>MSQSNRELVVDFLSYKLSQKGYSWSQFSDVEENRTEAPEGTESEAVKQALREAGDEFELRYRRAFSDLTSQLHITPGTAYQSFEQVVNELFRDGVNWGRIVAFFSFGGALCVESVDKEMQVLVSRIAAWMATYLNDHLEPWIQENGGWDTFVELYGNNAAAESRKGQERLEGGMA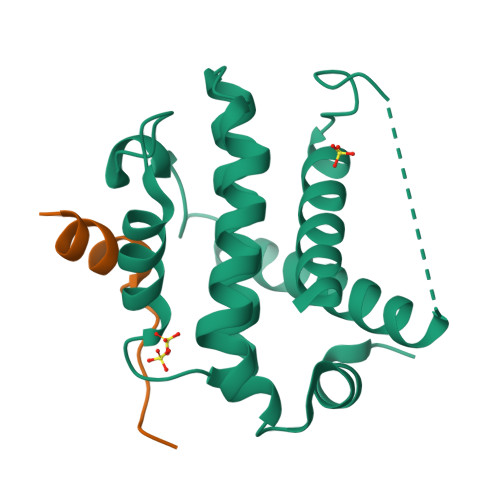VPPTYADLGKSARDVFTKGYGFGLGGHHHHHH[2x]> MGSMLSRSPVEPVQSTAPQPKAEPA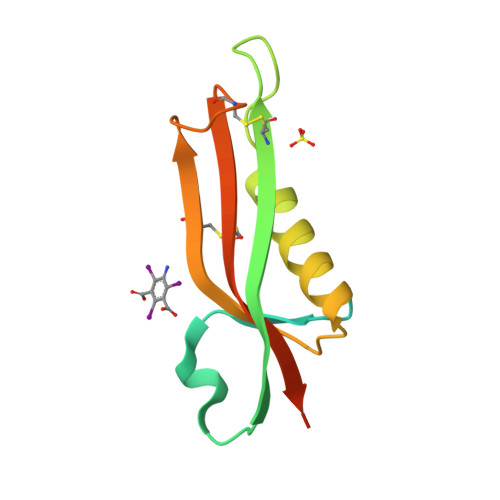KPKAPRATPVRIYTNAEELVGKPFRDLGEVSGDSCQASNQDSPPSIPTARKRMQINASKMKANAVLLHSCEVTSGTPGCYRQAVCIGSALNITAKLEHHHHHH>[2x]TRDFNGTWEMESNENFEGYMKALDIDFATRKIAVRLTFTDVIDQDGDNFKTKATST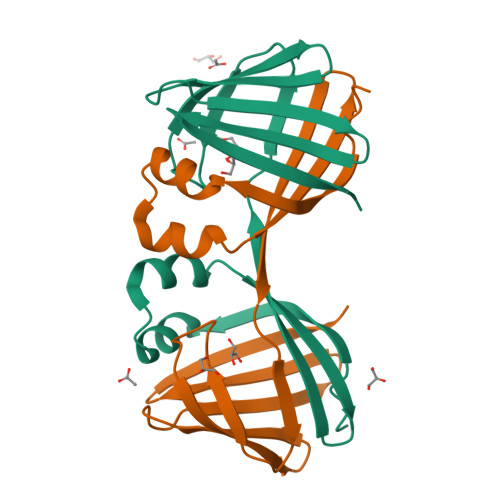HLNYDVDFTVGVEFDEYTKSLDNRHVKALVTWEGDVLVCVQKGEKENRGWKKWIEGDKLYLELTCGDQVCRQVFKKK>IEKKIVLRNGTEAFDSWEKPPLPVYTQFYFFNVTNPEEILRGETPRVEEVGPYTYRELRNKANIQFGDNGTTISAVSNKAYVFERDQSVGDPKIDLIRTLNIPVLTVIEWSQVHFLREIIEAMLKAYQQKLFVTHTVDELLWGYKDEILSLIHVFRPDISPYFGLFYEKNGTNDGDYVFLTGEDSYLNFTKIVEWNGKTSLDWWITDKCNMINGTDGDSFHPLITKDEVLYVFPSDFCRSVYITFSDYESVQGLPAFRYKVPAEILANTSDNAGFCIPEGNCLGSGVLNVSICKNGAPIIMSFPHFYQADERFVSAIEGMHPNQEDHETFVDINPL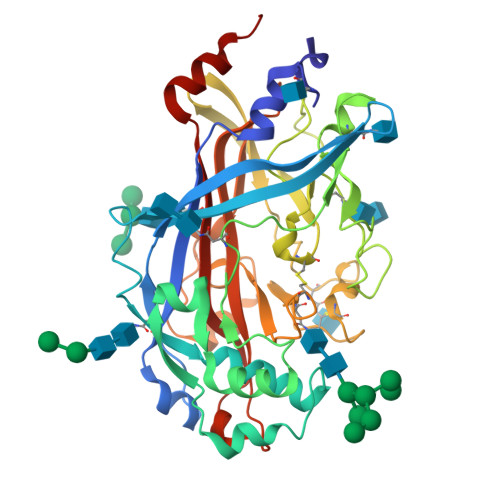TGIILKAAKRFQINIYVKKLDDFVETGDIRTMVFPVMYLNESVHIDKETASRLKSMIN[2x]> KIFKPEELRQALMPTLEALYRQDPESLPFRQPVDPQLLGIPDYFDI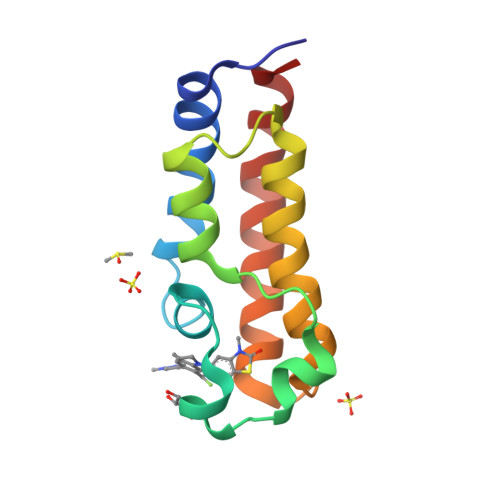VKNPMDLSTIKRKLDTGQYQEPWQYVDDVWLMFNNAWLYNRKTSRVYKFCSKLAEVFEQEIDPVMQSLG N-phenylcyclopropanecarboxamide 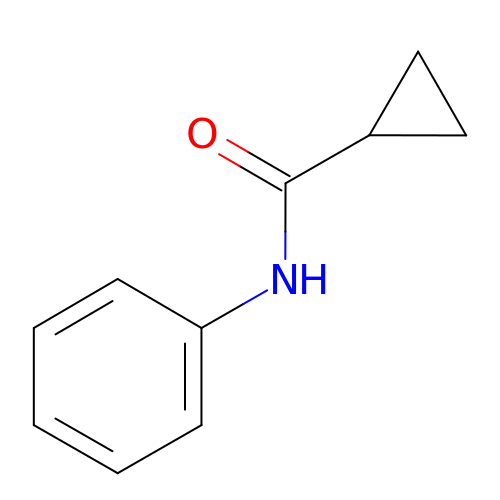| C10 H11 N O | OCHYJSATRBHPLB-UHFFFAOYSA-N>[2x]MKTIIINGVQFNTDEDTTILKFARDNNIDISALCFLNNCNNDINKCEICTVEVEGTGLVTACDTLIEDGMIINTNSDAVNEKIKSRISQLLDIHEFKCGPCNRRENCEFLKLVIKYKARASKPFLPKDKTEYVDERSKSLTVDRTKCLLCGRCVNACGKNTETYAMKFLNKNGKTIIGAEDEKCFDDTNCLLCGQCIIACPVAALSEKSHMDRVKNALNAPEKHVIVAMAPSVRASIGELFNMGFGVDVTGKIYTALRQLGFDKIFDINFGADMTIMEQATELVQRIENNGPFPMFTSCCPGWVRQAENYYPELLNNLSSAKSPQQIFGTASKTYYPSISGLDPKNVFTVTVMPCTSKKFEADRPQMEKDGLRDIDAVITTRELAKMIKDAKIPFAKLEDSEADPAMGEYSGAGAIFGATGGVMEAALRSAKDFAENAELEDIEYKQVRGLNGIKEAEVEINNNKYNVAVINGASNLFKFMKSGMINEKQYHFIEVMACHGGCVNGGGQPHVNPKDLEKVDIKKVRASVLYNQDEHLSKRKSHENTALVKMYQNYFGKPGEGRAHEILHFKYKKSAWSHPQFEK

[FeFe]-hydrogenases represent one of natures’ most effective classes of redox enzymes catalyzing the reversible reduction of protons to dihydrogen (H2) at turnover frequencies of up to 9000 s-11–3. With their low catalytic over-potential, [FeFe]-hydrogenases represent excellent models for a regenerative and likewise economically feasible H2 production. Their active center (“H-cluster”) can be structured into a standard [4Fe-4S]-cluster ([4Fe]H) and a diiron site ([2Fe]H). Theoretical studies suggest that the most probable PT pathway comprises of strictly conserved residues E282, S319, E279, and C299 (from surface to H-cluster, numbering corresponds to CpI), including two protein-bound water molecules (Wat826, Wat1120 4XDC19, chain B) located between E279 and C29915,16,20. In this study, site-directed mutagenesis (SDM) is used to investigate the PT pathway of two [FeFe]-hydrogenases, namely CpI and HydA1, which represent the largest (M3) and smallest (M1) type of monomeric [FeFe]-hydrogenases, respectively.

Corresponding to earlier crystal structure data, for all CpI variants a space group of P1 21 1 was observed with two copies in the asymmetric unit cell (chain A and B). The strongest impacts were achieved when replacing E279CpI for A or Q, or C299CpI for A or S, resulting in activities <1%. The conformational differences between E279QCpI and wild-type CpI are insignificant, except that the carboxamide group of Q279CpI is slightly twisted relative to the original carboxyl group. While glutamine occupies the entire space of the native carboxyl group and thus clearly interrupts the putative PT pathway, an exchange to alanine may support additional H2O molecules to bridge the gap. The conservative variant E279D retains 10–30% of H2 release activity but exhibits a significantly stronger down-shift in pH optimum than the largely inactive variant E279Q.>[4x]MRKIGIIGGTFDPPHYGHLLIANEVYHALNLEEVWFLPNQIPPHKQGRNITSVESRLQMLELATEAEEHFS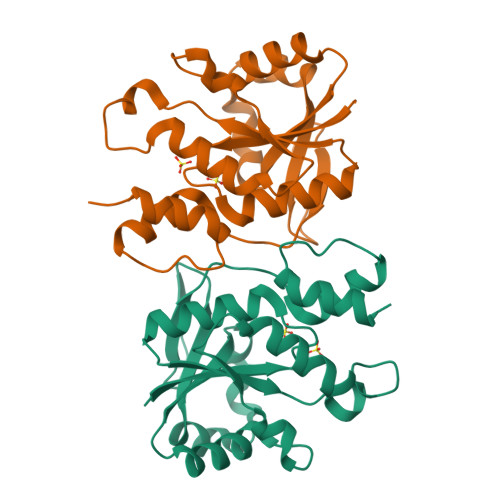ICLEELSRKGPSYTYDTMLQLTKKYPDVQFHFIIGGDMVEYLPKWYNIEALLDLVTFVGVARPGYKLRTPYPITTVEIPEFAVSSSLLRERYKEKKTCKYLLPEKVQVYIERNGLYESLAAALEHHHHHH>MQTEHVILLNAQGVPTGTLEKYAAHTADTRLHLAFSSWLFNAKGQLLVTRRALSKKAWPGVWTNSVCGHPQLGES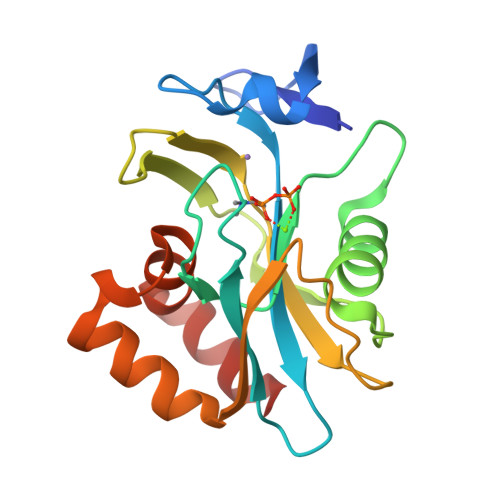NEDAVIRRCRYELGVEITPPESIYPDFRYRATDPSGIVENEVCPVFAARTTSALQINDDEVMDYQWCDLADVLHGIDATPWAFSPWMVMQATNREARKRLSAFTQLKL[2x]>[2x]FKIETTPESRYLAQIGDSVS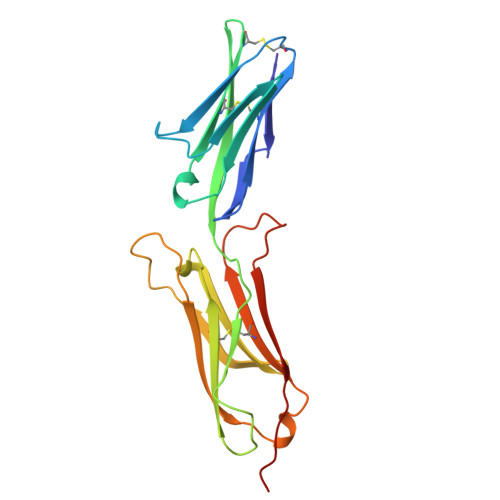LTCSTTGCESPFFSWRTQIDSPLNGKVTNEGTTSTLTMNPVSFGNEHSYLCTATCESRKLEKGIQVEIYSFPKDPEIHLSGPLEAGKPITVKCSVADVYPFDRLEIDLLKGDHLMKSQEFLEDADRKSLETKSLEVTFTPVIEDIGKVLVCRAKLHIDEMDSVPTVRQAVKELQVYISPKNT> AEPCDYPAQQLDLTDWKVTLPIGSSGKPSEIEQPALDTFATAPWFQVNAKCTGVQFRAAVNGVTTSGSGYPRSELREMTDGGEEKASWSATSGTHTMVFREAFNHLPEVKPHLVGAQIHDGDDDVTVFRLEGTSLYITKGDDTHHKLVTSDYKLNTVFEGKFVVSGGKIKVYYNGVLQTTISHTSSGNYFKAGAYTQ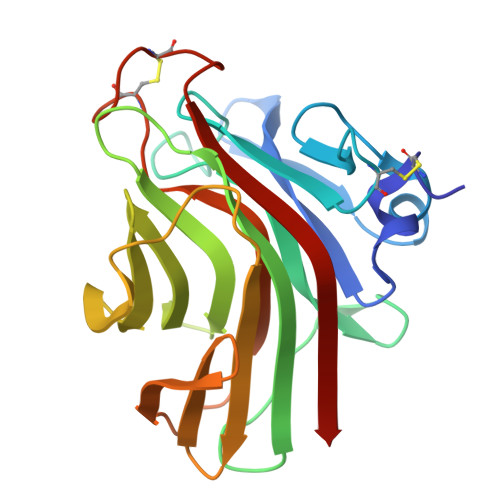ANCSNSSPCSSSNYGQVSLYKLQVTHS>[4x]GRKKRPLFPWFGLDIGGTLVKLVYFEPKDITAEEEEEEVESLKSIRKYLTSNVAYGSTGIRDVHLELKDLTLCGRKGNLHFIRFPTHDMPAFIQMGRDKNFSSLHTVFCATGGGAYKFEQDFLTIGDLQLCKLDELDCLIKGILYIDSVGFNGRSQCYYFENPADSEKCQKLPFDLK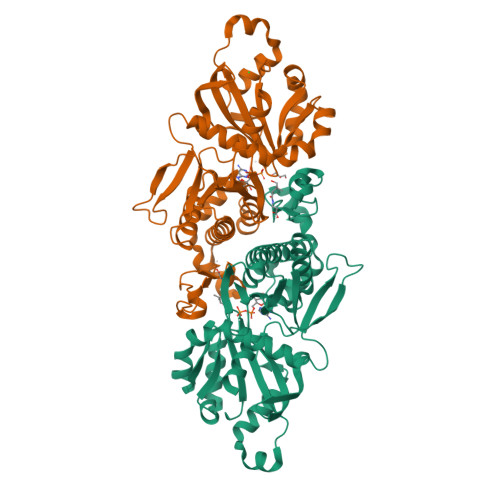NPYPLLLVNIGSGVSILAVYSKDNYKRVTGTSLGGGTFFGLCCLLTGCTTFEEALEMASRGDSTKVDKLVRDIYGGDYERFGLPGWAVASSFGNMMSKEKREAVSKEDLARATLITITNNIGSIARMCALNENINQVVFVGNFLRINTIAMRLLAYALDYWSKGQLKALFSEHEGYFGAVGALLELLK> MDSQGFWAILAFTPVLMILSLKGEGLLAMVGLLVLTVTLLASREKNDR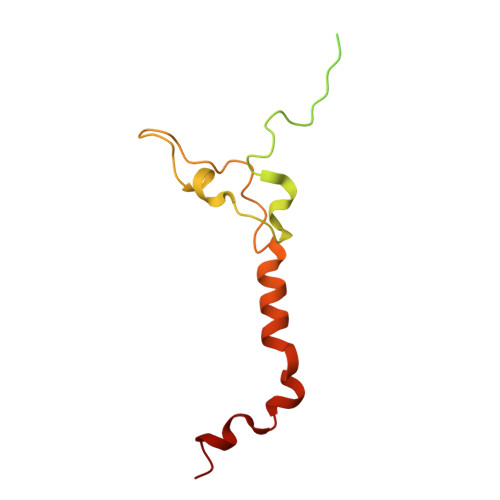PRLSCRGKIGRKVSGFENAGHVRDSHHVIYKRPPVNEYCAETREDNSLYVPEYCGQNWKNGVLSGMGTHHDAYRNLAVNMMTLRRESAVSAGWAHSYL> MPIKETDKEVVLTHPADETTSVHILKYGATVYSWKLKSEEQLWLSTAAKLDGSKPVRGGIPLVFPVFGKNSTDEH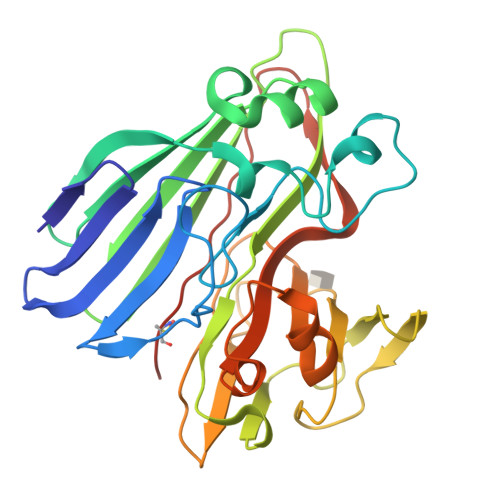LSKLPQHGLARNSTWEFLGQTKENPPTVQFGLKPEIANPELTKLWPMDYLLILTVELGSDYLKTAIEVENTSSSKELKFNWLFHTYFRIEDIEGTMVSNLAGMKLYDQLLKESYVDKHPVVTFNQETDVIYQNVSAERAIQIVDKGVQIHTLKRYNLPDTVVWNPWIEKSQGMADFEPKTGYQQMICIEPGHVHDFISLAPGKKWNAYQLLCKEELKYQAIQ>[2x]MPEISPHAPASADATRIAAIVAARQDIPGALLPILHEIQDTQGYIPDAAVPVIARALNLSRAEVHGVITFYHHFRQQPAGRHVVQVCRAEACQSVGAEALAEHAQRALGCGFHETTADGQVTLEPVYCLGQCACGPAVMVGEQLHGYVDARRFDALVRSLRESSAEKTTEAAEAQA;>[2x]MITITTIFVPRDSTALALGADDVARAIAREAAARNEHVRIVRNGSRGMFWLEPLVEVQTGAGRVAYGPVSAADVPGLFDAGLLQGGEHALSQGVTEEIPFLKQQERLTFARVGITDPLSLDDYRAHEGFAGLERALAMQPAEIVQEVTDSGLRGRGGAAFPTGIKWKTVLGAQSAVKYIVCNADEGDSGTFSDRMVMEDDPFMLIEGMTIAALAVGAEQGYIYCRSEYPHAIAVLESAIGIANAAGWLGDDIRGSGKRFHLEVRKGAGA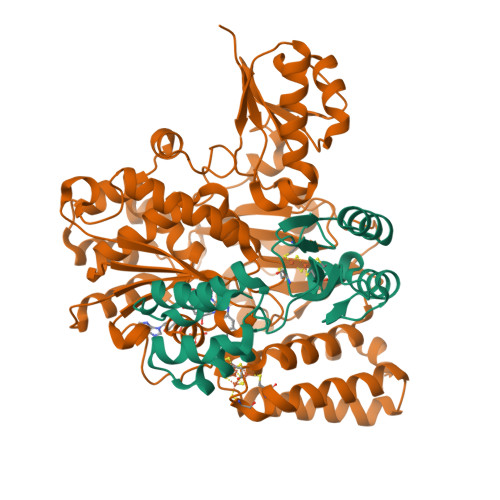YVCGEETALLESLEGRRGVVRAKPPLPALQGLFGKPTVINNVISLATVPVILARGAQYYRDYGMGRSRGTLPFQLAGNIKQGGLVEKAFGVTLRELLVDYGGGTRSGRAIRAVQVGGPLGAYLPESRFDVPLDYEAYAAFGGVVGHGGIVVFDETVDMAKQARYAMEFCAIESCGKCTPCRIGSTRGVEVMDRIIAGEQPVKHVALVRDLCDTMLNGSLCAMGGMTPYPVLSALNEFPEDFGLASNPAKAA>[2x]MSLSTFNRIHLVVLDSVGIGAAPDANNFSNAGVPDGASDTLGHISKTVGLNVPNMAKIGLGNIPRDTPLKTVPAENHPTGYVTKLEEVSLGKDTMTGHWEIMGLNITEPFDTFWNGFPEEIISKIEKFSGRKVIREANKPYSGTAVIDDFGPRQMETGELIIYTSADPVL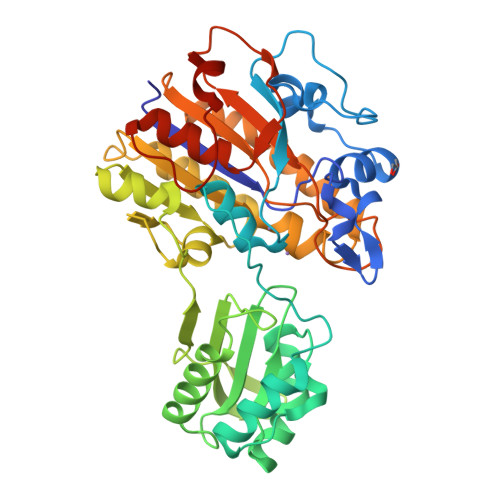QIAAHEDVIPLDELYRICEYARSITLERPALLGRIIARPYVGKPRNFTRTANRHDYALSPFAPTVLNKLADAGVSTYAVGKINDIFNGSGITNDMGHNKSNSHGVDTLIKTMGLSAFTKGFSFTNLVDFDALYGHRRNAHGYRDCLHEFDERLPEIIAAMKVDDLLLITADHGNDPTYAGTDHTREYVPLLAYSPSFTGNGVLPVGHYADISATIADNFGVDTAMIGESFLDKLIEGHHHHHH>[6x]SSQQVWKLVIITEEILLKKVSKIIKEAGASGYTVLAAAGE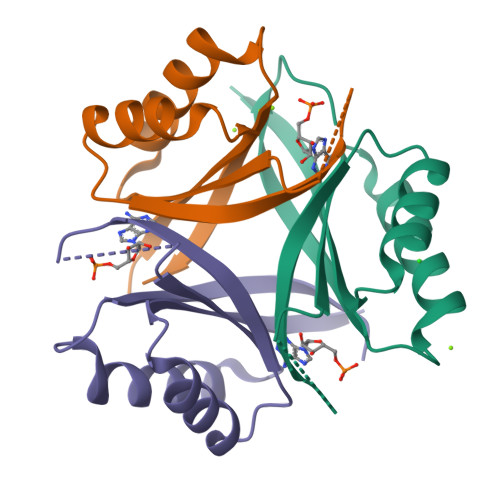GSRNVRSTGEPSVSHAYSNIKFEVLTASRELADQIQDKVVAKYFDDYSCITYISTVEALRAHKF>[3x]EMRIGHGFDVHAFGGEGPIIIGGVRIPYEKGLLAHSDGDVALHALTDALLGAAALGDIGKLFPDTDPAFKGADSRELLREAWRRIQAKGYTLGNVDVTIIAQAPK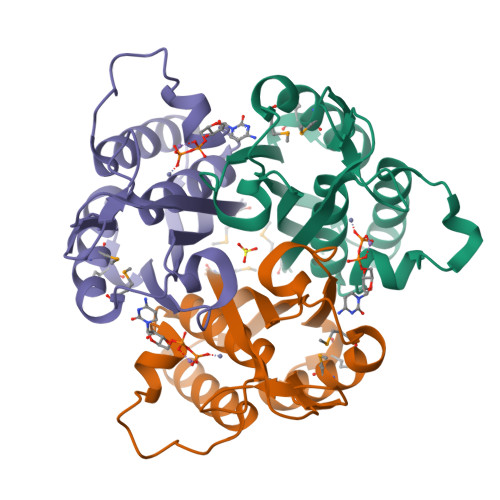MLPHIPQMRVFIAEDLGCHMDDVNVKATTTEKLGFTGRGEGIACEAVALLIKATK> MIGGLFIYNHKGEVLISRVYRDDIGRNAVDAFRVNVIHARQQVRSPVTNIARTSFFHVKRSNIWLAAVTKQNVNAAMVFEFLYKMCDVMAAYFGKISEENIKNNFVLIYELLDEILDFGYPQNSETGALKTFITQQGIKSQHQTKEEQSQITSQVTGQIGWRREGIKYRRNELFLDVLESVNLLMSPQGQVLSAHVSGRVVMKSYLSGMPECKFGMNDKIVIEKQGKGTADETSKSGKQSIAIDDCTFHQCVRLSKFDSERSISFIPPDGEFELMRYRTTKDIILPFRVIPLVREVGRTKLEVKVVIKSNFKPSLLAQKIEVRIPTPLNTSGVQVICMKGKAKYKASENAIVWKIKRMAGMKESQISAEIELLPTNDKKKWARPPI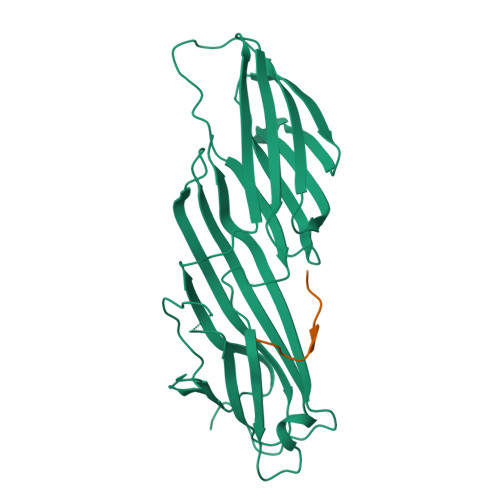SMNFEVPFAPSGLKVRYLKVFEPKLNYSDHDVIKWVRYIGRSGIYETRC;> VEDYEQGLSG> RKLILFIVFLALLLDNMLLTVVVPIIPSYLYSIKHEKNATEIQTARPVHTASISDSFQSIFSYYDNSTMVTGNATRDLTLHQTATQ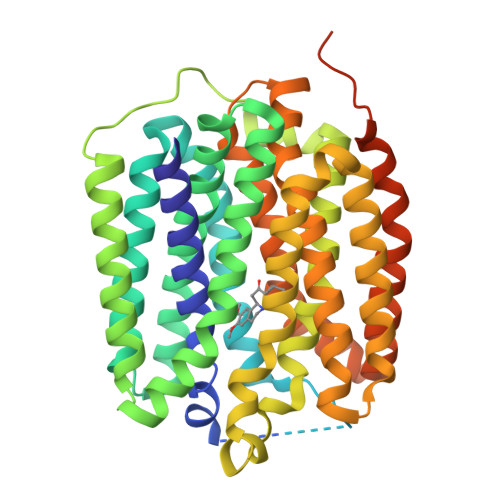HMVTNASAVPSDCPSEDKDLLNENVQVGLLFASKATVQLITNPFIGLLTNRIGYPIPIFAGFCIMFVSTIMFAFSSSYAFLLIARSLQGIGSSCSSVAGMGMLASVYTDDEERGNVMGIALGGLAMGVLVGPPFGSVLYEFVGKTAPFLVLAALVLLDGAIQLFVLQPSRVQPESQKGTPLTTLLKDPYILIAAGSICFANMGIAMLEPALPIWMMETMCSRKWQLGVAFLPASISYLIGTNIFGILAHKMGRWLCALLGMIIVGVSILCIPFAKNIYGLIAPNFGVGFAIGMVDSSMMPIMGYLVDLRHVSVYGSVYAIADVAFCMGYAIGPSAGGAIAKAIGFPWLMTIIGIIDILFAPLCFFLRSPPAKEEKMAILMDHNCPIKTKMYTQNNIQSYPIGEDEESESD ethyl 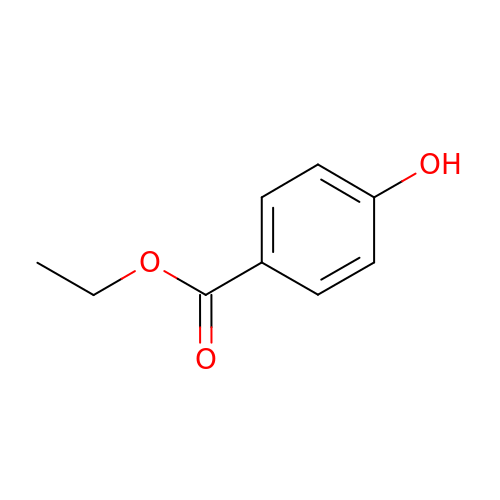4-hydroxybenzoate | C9 H10 O3 | NUVBSKCKDOMJSU-UHFFFAOYSA-N> SADAPVWID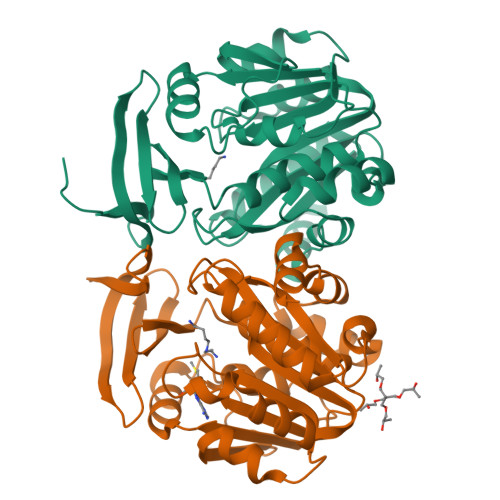EVFEDRVRYGLRGQILWEETSPFQKITIVDTEHYGRGLLLDDCWMTAERCEVCYHEYLVHPPLTTAASIARVLVIGGGDGGTVREVLRYAEVEQVDLVEIDGRVVELSQEYLGAIGTAWADPRLNVKIGDGIAFVQTAPDASYDVILVDGSDPAGGLFNREFYENCRRVLKPGGVFASQAESPDSFLAVHLEMIETLSAVFAEAKPYYGWVPMYPSGWWSWLYASDTPGQFQKPQSDRLAAIEPQVEIYNRDIHQAAFAQPNFVRRGLSARQ;> PVWIDEVFEDRVRYGLRGQILWEETSPFQKITIVDTEHYGRGLLLDDCWMTAERCEVCYHEYLVHPPLTTAASIARVLVIGGGDGGTVREVLRYAEVEQVDLVEIDGRVVELSQEYLGAIGTAWADPRLNVKIGDGIAFVQTAPDASYDVILVDGSDPAGPAAGLFNREFYENCRRVLKPGGVFASQAESPDSFLAVHLEMIETLSAVFAEAKPYYGWVPMYPSGWWSWLYASDTPGQFQKPQSDRLAAIEPQVEIYNRDIHQAAFAQPNFVRRGLSARQ>[2x]EEFDCHFLDEGFTAKDILDQKINEVSSSDDKDAFYVADLGDILKKHLRWLKALPRVTPFYAVKCNDSKAIVKTLAATGTGFDCASKTEIQLVQSLGVPPERIIYANPCKQVSQIKYAANNGVQMMTFDSEVELMKVARAHPKAKLVLRIATDDSKAVCRLSVKFGATLRTSRLLLERAKE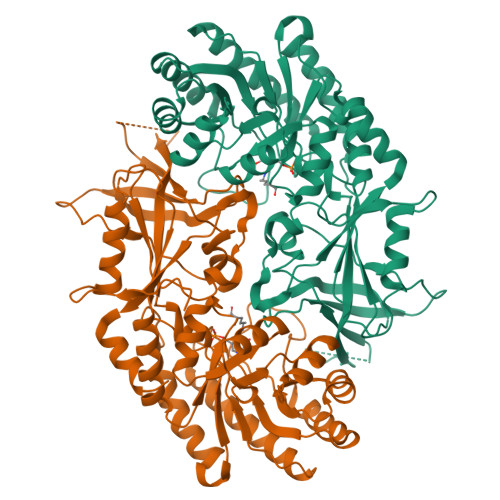LNIDVVGVSFHVGSGCTDPETFVQAISDARCVFDMGAEVGFSMYLLDIGGGFPGSEDVKLKFEEITGVINPALDKYFPSDSGVRIIAEPGRYYVASAFTLAVNIIAKKIVLKEQTGSDDEDESSEQTFMYYVNDGVYGSFNCILYDHAHVKPLLQKRPKPDERYYSSSIWGPTCDGLDRIVERCDLPEMHVGDWMLFENMGAYTVAAASTFNGFQRPTIYYVMSGPAWQLMQQFQNPDFPP>MHHHHHHSSGRENLYFQGSHKGSLQEVIGWGLIGWKYYANVIGPIQCEGLANLGVTQIACAEKRFLILSRNGRVYTQAYNSDTLAPQLVQGLASRNIVKIAAHSDGHHYLALAATGEVYSWGCGDGGRLGHGDTVPLEEPKVISAFSGKQAGKHVVHIACGSTYSAAITAEGELYTWGRGNYGRLGHGSSEDEAIPMLVAGLKGLKVIDVACGSGDAQTLAVTENGQVWSWGDGDYGKLGRGGSDGCKTPKLIEKLQDLDVVKVRCGSQFSIALTKDGQVYSWGKGDNQRLGHGTEEHVRYPKLLEGLQGKKVIDVAAGSTHCLALTEDSEVHSWGSNDQCQHFDTLRVTKPEPAALPGLDTKHIVGIACGPAQSFAWSSCSEWSIG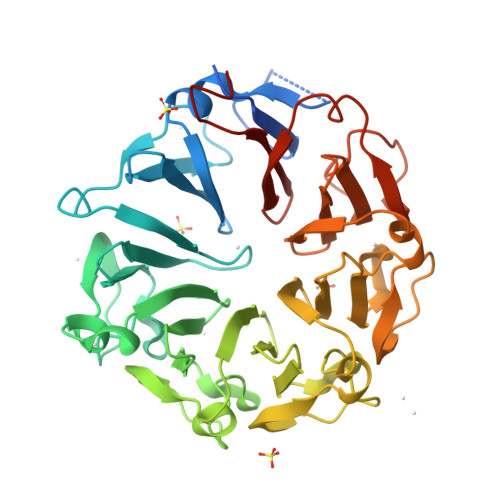LRVPF[3x]>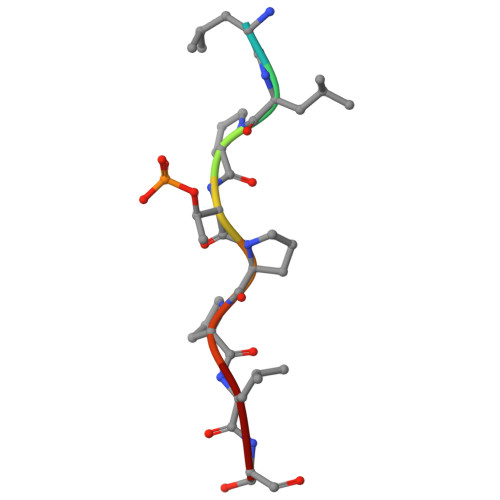 KLLPTPPLS>MSLIWKRKITLEALNA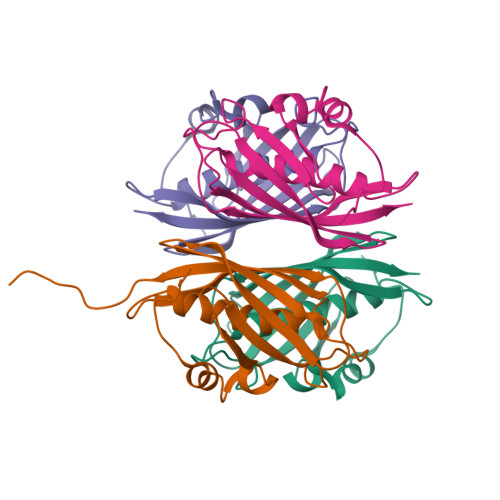MGEGNMVGFLDIRFEHIGDDTLEATMPVDSRTKQPFGLLHGGASVVLAESIGSVAGYLCTEGEQKVVGLEINANHVRSAREGRVRGVCKPLHLGSRHQVWQIEIFDEKGRLCCSSRLTTAILEGGSHHHHHH[8x]[(1S)-1-methyl-6-(7H-pyrrolo[2,3-d]pyrimidin-4-yl)-2,3-dihydro-1H-inden-1-yl]cyanamide | C17 H15 N5 | 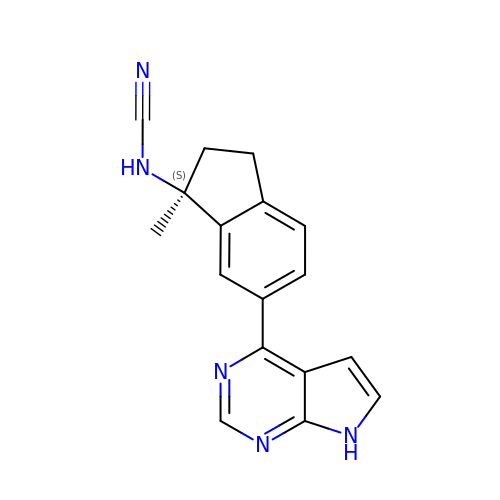PTCVBQDKOCSZKC-KRWDZBQOSA-N>RHMKVLLLGFEFLPVKVGGLAEALTAISEALASLGHEVLVFTPSHGRFQGEEIGKIRVFGEEVQVKVSYEERGNLRIYRIGGGLLDSEDVYGPGWDGLIRKAVTFGRASVLLLNDLLREEPLPDVVHFHDWHTVFAGALIKKYFKIPAVFTIHRLNKSKLPAFYFHEAGLSELAPYPDIDPEHTGGYIADIVTTVSRGYLIDEWGFFRNFEGKITYVFNGIDCSFWNESYLTGSRDERKKSLLSKFGMDEGVTFMFIGRFDRGQKGVDVLLKAIEILSSKKEFQEMRFIIIGKGDPELEGWARSLEEKHGNVKVITEMLSREFVRELYGSVDFVI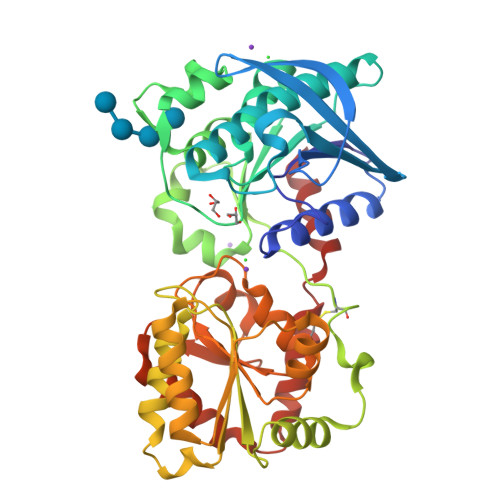IPSYFEPFGLVALEAMCLGAIPIASAVGGLRDIITNETGILVKAGDPGELANAILKALELSRSDLSKFRENCKKRAMSFSWEKSAERYVKAYA[2x]KLHL3 is the substrate-recognition subunit of the ubiquitin ligase complex, recruiting substrates for ubiquitylation via its associated Kelch domain. KLHL2 shares 84% sequence identity with KLHL3 across the Kelch domain, and 86% identity overall. KLHL2 has also been implicated recently as a CUL3 substrate adaptor for WNK kinases. We determined the high-resolution crystal structures of the Kelch domains of human KLHL3 and KLHL2 in separate complexes with the 11-residue WNK4 degron motif.

Two Kelch domains were found in the asymmetric unit of each structure. The KLHL2 structure was solved at 1.6 Å (1 Å=0.1 nm) resolution in space group P43212, whereas the structure of KLHL3 was determined at 1.8 Å in space group P212121. The KLHL2 and KLHL3 structures were determined at pH 7.5 and pH 4.3 respectively, which probably contributes to differences in the resolution of particular residues. For the KLHL2 structure, residues 292–305 from the N-terminus and residues 592–593 from the C-terminus were not clearly resolved in the electron density and were excluded from the model, as was the C-terminal residue of the WNK4 peptide (Gln567). WNK4 Gln567 was disordered in both structures, consistent with a lack of stabilizing side-chain contacts, yet was critical for peptide binding. The presented structures reveal that KLHL2 and KLHL3 bind to the WNK1/4 degron in an almost indistinguishable manner and maintain strict conservation of all critical contact residues. Consistent with this, we found that the WNK1/4 degron motif bound to the Kelch domain of KLHL2 with similar affinity to KLHL3. Our data further support the recent finding that KLHL2 may also function as a second CUL3 adaptor for the WNK kinases. Thus far, no mutations in KLHL2 have been described in patients with Gordon's syndrome, but the binding data strongly suggest that KLHL2 will also play a role in regulating WNK isoforms. KLHL2 is best known for its high expression in the brain, whereas KLHL3 may play a dominant role in the kidney, consistent with the effects of KLHL3 mutations in hypertension.

>[2x]SMSVRTRLRTPMNLPKLMVVVGGQAPKAIRSVECYDFKEERWHQVAELPSRRCRAGMVYMAGLVFAVGGFNGSLRVRTVDSYDPVKDQWTSVANMRDRRSTLGAAVLNGLLYAVGGFDGSTGLSSVEAYNIKSNEWFHVAPMNTRRSSVGVGVVGGLLYAVGGYDVASRQCLSTVECYNATTNEWTYIAEMSTRRSGAGVGVLNNLLYAVGGHDGPLVRKSVEVYDPTTNAWRQVADMNMCRRNAGVCAVNGLLYVVGGDDGSCNLASVEYYNPTTDKWTVVSSCMSTGRSYAGVTVIDKRL;>EPEEPEADQHQ[2x]> MDALLTKFNEDRSLQDENLSQPRTRVRIVDDNLYNKSNPFQLCYKKRDYGSQYYHIYQYRLKTFRERVLKECDKRWDAGFTLNGQLVLKKDKVLDIQGNQPCWCVGSIYCEMKYKPNVLDEVINDTYGAPDLTKSYTDKEGGSDEIMLEDESGRVLLVGDFIRSTPFITGVVVGILGMEAEAGTFQVLDICYPTPLPQNPFPAPIATCPTRGKIALVSGLNLNNTSPDRLLRLEILREFLMGRINNKIDDISLIGRLLICGNSVDFDIKSVNKDELMISLTEFSKFLHN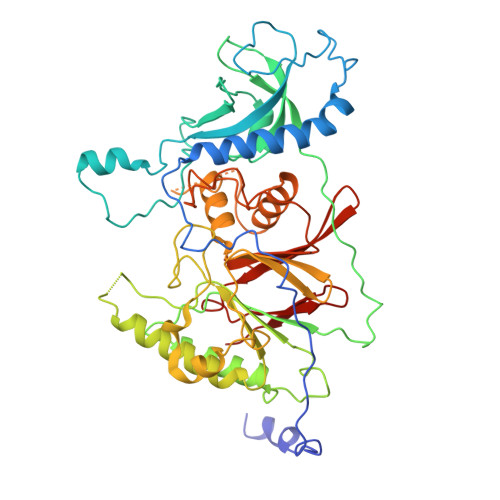ILPSISVDIMPGTNDPSDKSLPQQPFHKSLFDKSLESYFNGSNKEILNLVTNPYEFSYNGVDVLAVSGKNINDICKYVIPSNDNGESENKVEEGESNDFKDDIEHRLDLMECTMKWQNIAPTAPDTLWCYPYTDKDPFVLDKWPHVYIVANQPYFGTRVVEIGGKNIKIISVPEFSSTGMIILLDLETLEAETVKIDI Guanine-rich DNAs can fold into noncanonical DNA structures called G-quadruplexes (G4s). The highly stable G4s can impede many cellular processes such as replication, transcription, and translation, and the failure to resolve G4s results in genome instability. Pif1 helicase binds preferentially to G4 DNA and plays multiple roles in maintaining genome stability, but the mechanism by which Pif1 unfolds G4s is poorly understood. Pif1 helicase plays multiple roles in maintaining genome stability in both the nucleus and mitochondria.

We then went on to crystallize ScPif1 in complex with ADP·AlF4− and T7-AT11 containing a 5′ T7 ssDNA loading site (designated as ScPif1-G4) and determined its structure at a resolution of 3.5 Å. The asymmetric unit of the crystal structure contains two essentially identical ScPif1-G4 complexes. The AT11 portion of the DNA substrate is well ordered in the electron density map and adopts a G4 conformation very similar to that of AT11 alone, indicating that ScPif1 did not disrupt the G4 structure. In the structure of ScPif1-G4, the conformation of ScPif1 is very similar to that of ScPif1 bound to a ssDNA29 except for the 2B domain, which rotates 9° upon G4 binding relative to ssDNA bound ScPif1. ScPif1 recognizes G4 mainly through the wedge region containing α5 and α6 with additional interactions contributed by the β15-β16 loop in the 2B domain. The prominent feature of the ScPif1-G4 interactions is that R324 interacts with G12 in the 5′ most G-tetrad (G9.G12.G15.G19) through cation-π interaction and with T8 (the first nucleotide preceding the 5′ most G-tetrad) through van der Waals contacts, which in turn stacks against G9. Additional interactions involve R326 which contacts the phosphate backbone between G9 and G10 and the base of T11, and R323, which interacts with the phosphate backbone connecting T11 and G12, and L329 and R330, which interact with the base of T11 through van der Waals contacts. Compared with the wedge region, the β15-β16 loop in the 2B domain interacts solely with the peripheral region of the G4 and has no contact with the G-tetrad. In the structure of ScPif1-G4, the Pif1 signature motif not only contacts the regions involved in ssDNA binding but also interacts with the two α-helices in the wedge region predominantly through extensive hydrophobic contacts, thereby stabilizing the wedge region. Our ScPif1-G4 structure showed that the structurally conserved wedge region contacts the ssDNA/G4 junction with R324 playing a key role in mediating the interaction of ScPif1 with G4.

>[2x]CLSKEQESIIKLAENGHNIFYTGSAGTGKSILLREMIKVLKGIYGRENVAVTASTGLAACNIGGITIHSFAGIGLGKGDADKLYKKVRRSRKHLRRWENIGALVVDEISMLDAELLDKLDFIARKIRKNHQPFGGIQLIFCGDFFQLPPVSKDPNRPTKFAFESKAWKEGVKMTIMLQKVFRQRGDVKFIDMLNRMRLGNIDDETEREFKKLSRPLPDDEIIPAELYSTRMEVERANNSRLSKLPGQVHIFNAIDGGALEDEELKERLLQNFLAPKELHLKVGAQVMMVKNLDATLVNGSLGKVIEFMDPETYFCYEALTNDPSMPPEKLETWAENPSKLKAAMEREQSDGEESAVASRKSSVKEGFAKSDIGEPVSPLDSSVFDFMKRVKTDDEVVLENIKRKEQLMQTIHQNSAGKRRLPLVRFKASDMSTRMVLVEPEDWAIEDENEKPLVSRVQLPLMLAWSLSIHKSQGQTLPKVKVDLRRVFEKGQAYVALSRAVSREGLQVLNFDRTRIKAHQKVIDFYLTLSSAESAYKQLEADEQV> ASAPIGSAISRNNWAVTCDSAQSGNECNKAIDGNKDTFWHTFYGANGDPKPPHTYTIDMKTTQNVNGLSMLPRQDGNQNGWIGRHEVYLSSDGTNWGSPVASGSWFADSTTKYSNFETRPARYVRLVAITEANGQPWTSIAEINVFQASSYTAPQPGLGRWGPTIDLPIVPAAAAIEPTSGRVLMWSSYRNDAFGGSPGGITLTSSWDPSTGIVSDRTVTVTKHDMFCPGISMDGNGQIVVTGGNDAKKTSLYDSSSDSWIPGPDMQVARGYQSSATMSDGRVFTIGGSGSGGVFEKNGEVYSPSSKTWTSLPNAKVNPMLTADKQGL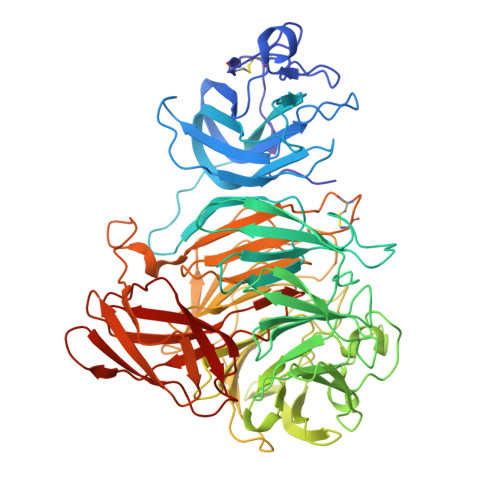YRSDNHAWLFGWKKGSVFQAGPSTAMNWYYTSGSGDVKSAGKRQSNRGVAPDAMCGNAVMYDAVKGKILTFGGSPDYQDSDATTNAHIITLGEPGTSPNTVFASNGLYFARTFHTSVVLPDGSTFITGGQRRGIPFEDSTPVFTPEIYVPEQDTFYKQNPNSIVRVYHSISLLLPDGRVFNGGGGLCGDCTTNHFDAQIFTPNYLYNSNGNLATRPKITRTSTQSVKVGGRITISTDSSISKASLIRYGTATHTVNTDQRRIPLTLTNNGGNSYSFQVPSDSGVALPGYWMLFVMNSAGVPSVASTIRVTQ> SMAAFKPNSINYILGLDIGIASVGWAMVEIDEEENPIRLIDLGVRVFERAEVPKTGDSLAMARRLARSVRRLTRRRAHRLLRTRRLLKREGVLQAANFDENGLIKSLPNTPWQLRAAALDRKLTPLEWSAVLLHLIKHRGYLSQRKNEGETADKELGALLKGVAGNAHALQTGDFRTPAELALNKFEKESGHIRNQRSDYSHTFSRKDLQAELILLFEKQKEFGNPHVSGGLKEGIETLLMTQRPALSGDAVQKMLGHCTFEPAEPKAAKNTYTAERFIWLTKLNNLRILEQGSERPLTDTERATLMDEPYRKSKLTYAQARKLLGLEDTAFFKGLRYGKDNAEASTLMEMKAYHAISRALEKEGLKDKK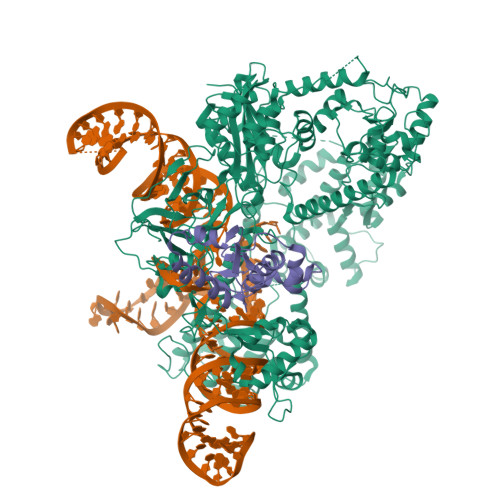SPLNLSPELQDEIGTAFSLFKTDEDITGRLKDRIQPEILEALLKHISFDKFVQISLKALRRIVPLMEQGKRYDEACAEIYGDHYGKKNTEEKIYLPPIPADEIRNPVVLRALSQARKVINGVVRRYGSPARIHIETAREVGKSFKDRKEIEKRQEENRKDREKAAAKFREYFPNFVGEPKSKDILKLRLYEQQHGKCLYSGKEINLGRLNEKGYVEIDHALPFSRTWDDSFNNKVLVLGSENQNKGNQTPYEYFNGKDNSREWQEFKARVETSRFPRSKKQRILLQKFDEDGFKERNLNDTRYVNRFLCQFVADRMRLTGKGKKRVFASNGQITNLLRGFWGLRKVRAENDRHHALDAVVVACSTVAMQQKITRFVRYKEMNAFDGKTIDKETGEVLHQKTHFPQPWEFFAQEVMIRVFGKPDGKPEFEEADTLEKLRTLLAEKLSSRPEAVHEYVTPLFVSRAPNRKMSGQGHMETVKSAKRLDEGVSVLRVPLTQLKLKDLEKMVNREREPKLYEALKARLEAHKDDPAKAFAEPFYKYDKAGNRTQQVKAVRVEQVQKTGVWVRNHNGIADNATMVRVDVFEKGDKYYLVPIYSWQVAKGILPDRAVVQGKDEEDWQLIDDSFNFKFSLHPNDLVEVITKKARMFGYFASCHRGTGNINIRIHDLDHKIGKNGILEGIGVKTALSFQKYQIDELGKEIRPCRLKKRPPVR;> SMNNSIKFHVSYDGTARALFNTKEQAEKYCLVEEINDEMNGYKRKSWEEKLREENCASVQDWVEKNYTSSYSDLFNICEIEVSSAGQLVKIDNTEVDDFVENCYGFTLEDDLEEFNKAKQYLQKFYAECEN>MRGSHHHHHHGSSGLLKESMRIKMYMEGTVNGHYFKCEGEGDGNPFAGTQSMRIHVTEGAPLPFAFDILAPCCEYGSRTFVHHTAEIPDFFKQSFPEGFTWERTTTYEDGGILTAHQDTSLEGNCLIYKVKVLGTNFPADGPVMKNKSGGWEPSTEVVYPENGVLCGRNVMALKVGDRRLICHHYTS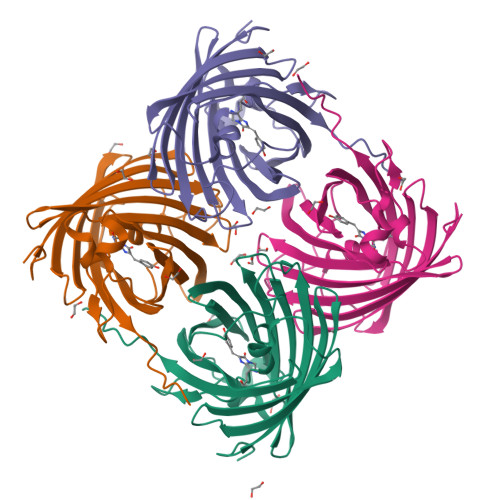YRSKKAVRALTMPGFHFTDIRLQMLRKEKDEYFELYEASVARYSDLPEKAN[4x]> MASMPSRTALSPGVLSPTRPVPNWIARPEYVGKPAAQEGSEPWVQTPEVIEKMRVAGRIAAGALAEAGKAV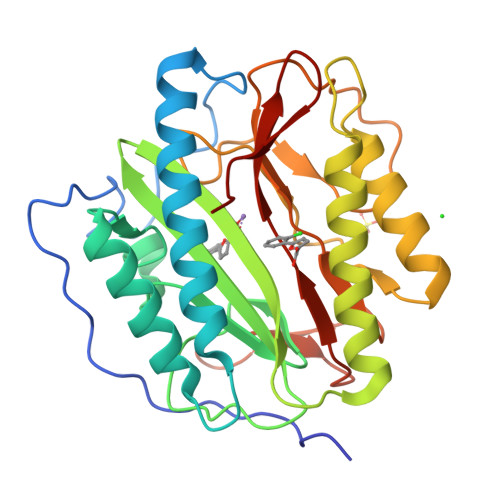APGVTTDELDRIAHEYLVDNGAYPSTLGYKGFPKSCCTSLNEVICHGIPDSTVITDGDIVNIDVTAYIGGVHGDTNATFPAGDVADEHRLLVDRTREATMRAINTVKPGRALSVIGRVIESYANRFGYNVVRDFTGHGIGTTFHNGLVVLHYDQPAVETIMQPGMTFTIEPMINLGALDYEIWDDGWTVVTKDRKWTAQFEHTLLVTDTGVEILTCL> GNRVIDAEPREIPLEYADDLLEAMAHHRPV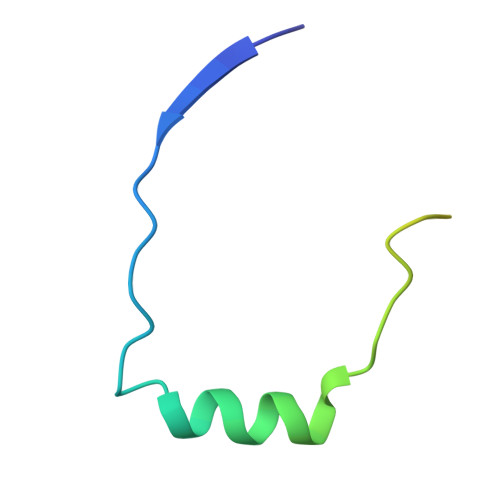PCSLGLSQAIANNTPIQQISETFWKYRK>LQFYRNLGKSGLRVSCLGLGTWVTFGGQITDEMAEHLMTLAYDNGINLFDTAEVYAAGKAEVVLGNIIKKKGWRRSSLVITTKIFWGGKAETERGLSRKHIIEGLKASLERLQLEYVDVVFANRPDPNTPMEETVRAMTHVINQGMAMYWGTSRWSSMEIMEAYSVARQFNLIPPICEQAEYHMFQREKVEVQLPELF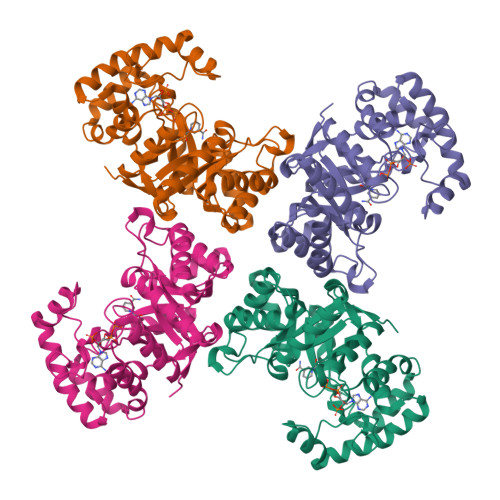HKIGVGAMTWSPLACGIVSGKYDSGIPPYSRASLKGYQWLKDKILSEEGRRQQAKLKELQAIAERLGCTLPQLAIAWCLRNEGVSSVLLGASNAEQLMENIGAIQVLPKLSSSIVHEIDSILGNKPY[4x]> SSDRPRGRDPVNPEKLLVITVATAETEGYLRFLRSAEFFNYTVRTLGLGEEWRGGDKARTVGGGQKVRWLKKEMEKYADREDMIIMFVDSYDVILAGSPTELLKKFVQSGSRLLFSAESFCWPEWGLAEQYPEVGTGKRFLNSGGFIGFATTIHQIVRQWKYKDDDDDQLFYTRLYLDPGLREKLSLNLDHKSRIFQNLNGALDEVVLKFDRNRVRIRNVAYDTLPIVVHGNGPTKLQLNYLGNYVPNGWTPEGGCGFCNQDRRTLPGGQPPPRVFLAVFVEQPTPFLPRFLQRLLLLDYPPDRVTLFLHNNEVFHEPHIADSWPQLQDHFSAVKLVGPEEALSPGEARDMAMDLCRQDPECEFYFSLDADAVLTNLQTLRILIEENRKVIAPMLSRHGKLWSNFWGALSPDEYYARSEDYVELVQRKRVGVWNVPYISQAYVIRGDTLRMELPQRDVFSGSDTDPDMAFCKSFRDKGIFLHLSNQHEFGRLLATSRYDTEHLHPDL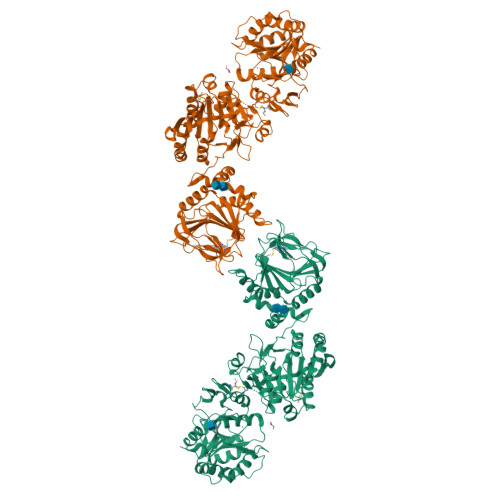WQIFDNPVDWKEQYIHENYSRALEGEGIVEQPCPDVYWFPLLSEQMCDELVAEMEHYGQWSGGRHEDSRLAGGYENVPTVDIHMKQVGYEDQWLQLLRTYVGPMTESLFPGYHTKARAVMNFVVRYRPDEQPSLRPHHDSSTFTLNVALNHKGLDYEGGGCRFLRYDCVISSPRKGWALLHPGRLTHYHEGLPTTWGTRYIMVSFVDPAAA>[2x]MGIRITGTGLFHPTEIISNEELADSLNAYVEQYNQENAEKIAAGELEELRGSSAEFIEKASGIKRRYVIEKSGILDPTRLRPRLSERSNDELSIQAEWGVIAAKQAMENAGVTAEDIDVVILACSNMQRAYPAVAIEIQSALGIQG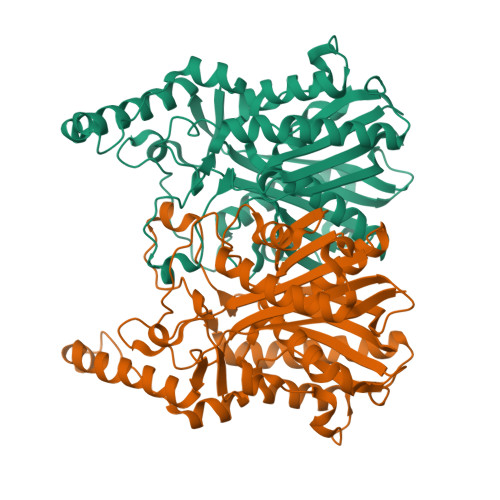YAYDMNVACSAATFGLKQAADAIRSGARRVLLVNVEITSGHLDYRNRDCHFIFGDVATASIIEETTTKTGFEILDIHLFTQFSNNIRNNFGFLNRSEDAVVDDKLFRQDGRKVFKDVCPLVAKIINAQLEKMQLTANDIKRFWLHQANANMNELILKYVAGKDADLSRAPIILDEFANTSSAGVIIALHRTGHEVDDGEYGVISSFGAGYSVGSIVVQKHVA>[2x]GSHMPNYKLTYFNMRGRAEIIRYIFAYLDIQYEDHRIEQADWPEIKSTLPFGKIPILE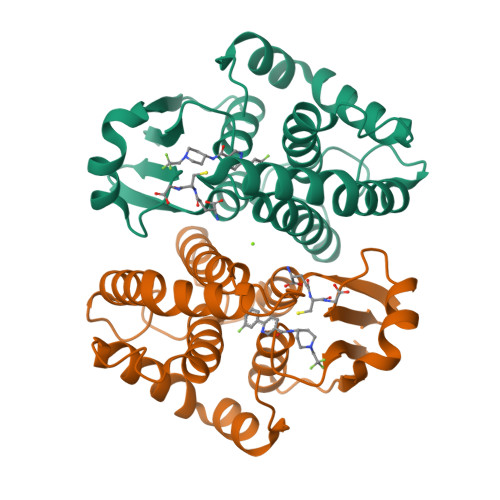VDGLTLHQSLAIARYLTKNTDLAGNTEMEQCHVDAIVDTLDDFMSCFPWAEKKQDVKEQMFNELLTYNAPHLMQDLDTYLGGREWLIGNSVTWADFYWEICSTTLLVFKPDLLDNHPRLVTLRKKVQAIPAVANWIKRRPQTKL To gain insight into the evolution and designability of ligand binding and specificity, we analyzed the homologous PBPs, PotF and PotD, which are Escherichia coli putrescine (PUT)-binding protein and spermidine (SPD)-binding protein, respectively. They constitute the first elements of two separate multicomponent uptake systems (PotFGHI and PotABCD) to transport the cationic polyamines PUT and SPD across the cellular membrane. Still, the protein-binding modes differ: PotF shows affinity for PUT and SPD, whereas PotD exclusively binds SPD. Prior to this work, we grafted the seven differences in amino acids from PotD binding pocket onto PotF; this resulted in PotF_SPD, which will be referred to as PotF/D throughout this work to keep naming for mutants more concise.

Unfortunately, we were not able to crystallize F88A after numerous attempts, while high-resolution structures for both other variants were acquired. It seemed the removal of a whole benzene ring in F88A and keeping only a methyl group destabilized the protein by creating a large unoccupied space. To counteract the aforementioned difficulties, we constructed a variant bearing F88L instead of F88A. It acts as a substitute to evaluate whether the structural positioning of Y87 can be altered by removing F88. We obtained high-resolution datasets for this variant in a similar fashion as for the other constructs. To our surprise, all solved structures adopt a PotF/D-like semiclosed conformation. The same behavior is observed in the F88L variant where Leu tries to mimic Phe positioning. In F88L, Y87 remains flipped outside the distal region of the binding pocket. Tyr fills the unoccupied space between the salt bridge residues, interacts with R91 of the salt bridge, and stacks with Q348.

> AEQKTLHIYNWTDYIAPDTVANFEKETGIKVVYDVFDSNEVLEGKLMAGSTGFDLVVPSAYLLERQLTAGVFQPLDKSKLPEWKNLDPELLKLVAKHDPDNKFAMPYMWATTGIGYNVDKVKAVLGENAPVDSWDLILKPENLEKLKSCGVSFLDDPEEVFATVLNYLGKDPNSTKADDYTGPATDLLLKLRPNIRYFHSSQYINDLANGDICVAIGWAGSVWQASNRAKEAKNGVNVSFSIPKEGAMAWFDVFAMPADAKNKDEAYQFLNYLLRPDVVAHISDHVFYANANKAATPLVSAEVRENPGIYPPADVRAKLFTQKVQDPKIDRVRTRAWTKVKSGKLEHHHHHH> MKNWKTSAESILTTGPVVPVIVVKKLEHAVPMAKALVAGGVRVLNVTLRTECAVDAIRAIAKEVPEAIVGAGTVLNPQQLAEVTEAGAQFAISPGLTEPLLKAATEGTIPLIPGISTVSELMLGMDYGLKEFKFFPAEANGGVKALQAIAGPFSQVRFCPTGGISPANYRD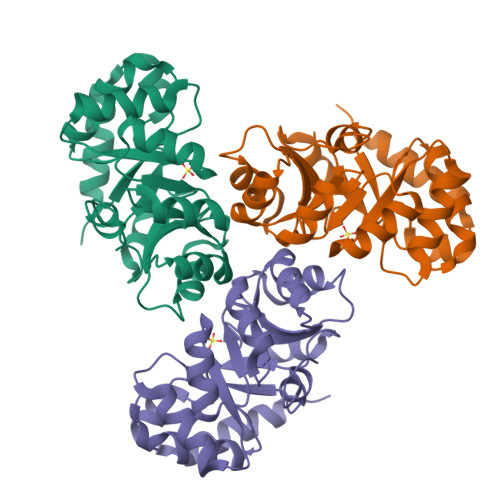YLALKSVLCIGGSWLVPADALEAGDYDRITKLAREAVEGAKL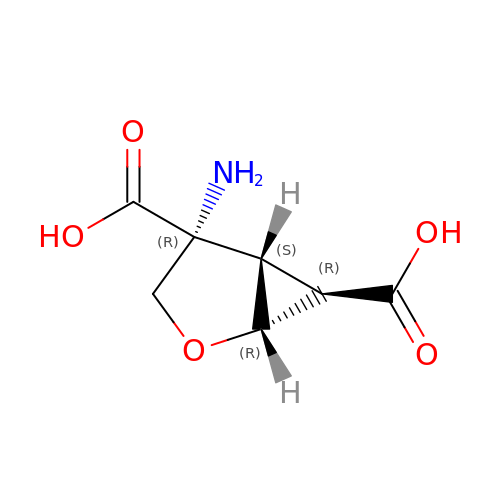(1R,4R,5S,6R)-4-azanyl-2-oxabicyclo[3.1.0]hexane-4,6-dicarboxylic acid | C7 H9 N O5 | YASVRZWVUGJELU-BXPDIHNCSA-N>MNHKVHHHHHHIEGRHMTNTRSAVVLGGGMAGMLVSSMLARHVGSVTVIDRDAFPAGPDLRKGVPQARHAHILWSGGARIVEELLPGTTDRLLGAGAHRIGIPDGQVSYTAYGWQHRFPEAQFMIACSRALLDWTVREETLREERIALVEKTEVLALLGDAGRVTGVRVRDQESGEEREVPADLVVDTMGRGSPMKRLLAELGLPAPEEEFVDSGMVYATRLFRAPEAAATNFPLVSVHADHRAGRPGCNAVLMPIEDGRWIVTVSGTRGGEPPADDEGFARFARDGVRHPLVGELIAXAQPLTSVERSRSTVNRRLHYDRLATWPEGLVVLGDAVAAFNPVYGHGMSAAAHSVLALRSQLGQRAFQPGLARAAQRAIAVAVDDAWVLATSHDIGYPGCRTQTRDPRLTRHAGERQRVTDLVGLTATRNQVVNRAAVALNTLSAGMASMQDPAVMAAVRRGPEVPAPTEPPLRPDEVARLVSGAGVTA[2x]

Lasalocid A, a polyether ionophore natural product derived from Streptomyces lasalocidi, is a widely used veterinary medicine that acts by transporting various cations across the cell membrane, thereby disrupting cation homeostasis. Lasalocid A biosynthesis entails two stereospecific epoxidation of the precursor diene, catalyzed by the flavin-dependent enzyme Lsd18. We performed protein engineering on Lsd18 to improve its thermostability and catalytic activity. Screening of these mutants using thermal shift assay identified stabilized variants Lsd18-T189M, Lsd18-S195M, and the double mutant Lsd18-T189M-S195M.

We found that the Tm values of Lsd18-T189M, Lsd18-S195M, and Lsd18-T189M-S195M were increased by 3.0 °C, 4.5 °C, and 4.8 °C, respectively. As expected, the FAD content in the mutants Lsd18-T189M, Lsd18-S195M, Lsd18-T189M-S195M increased by 29.3%, 46.7%, and 38.3%, respectively, compared to the wild-type Lsd18. The structural stability of the double-mutation system is lower than the S195M mutation system but higher than the T189M mutation system. In order to reveal the structural basis for the higher thermostability of the best two mutants, we solved the crystal structures of Lsd18-S195M and Lsd18-T189M-S195M at the resolution of 2.50 Å and 3.76 Å, respectively. Although the resolution of the second structure was not high, the secondary structure was clear enough for analysis. Comparing the structures of Lsd18 WT, Lsd18-S195M, and Lsd18-T189M-S195M, it can be seen that the angle of the α helix between L408 and T419 shifts, which is in agreement with the MD study. Furthermore, the loop region R314-L316, E208-F210 and C398-Q401 in Lsd18 WT change to a β sheet in the two mutants’ crystal structures, also indicating that this region is less flexible and more stable. T189 formed hydrogen bonds with D187 and G192. After mutating to M189, the hydrogen bond with G192 was weakened, while there were hydrophobic interactions between M189 and L26 as well as P194. More importantly, M189 forms a hydrogen bond with the cofactor FAD that could stabilize the binding of this cofactor.> MSSDLVMPALGRPFTLGMLYDARREKLIPGFSLFGDETLQKYQSSNAQRSSEFKIVASDSTESKSSAMDIEASLGVSFLGGLVEVGGSAKYLNNTKKYQNQSRVTLKYKATTVYKQFTAPPGTVTVQETAITEKGLATHVVTSILYGANAFFVSDSDKVEDTNLQDIQGKMEAAIKKIPTISIEGSASVQLTDEEKSLASNLSCKFHGDFLLESLPTTFEDAVKTYQTLPTLIGEDGANSVPMKVWLAPLKSYNSKAQQLIQEINVSKVRRIHTTLEELHKLKRRANEAMDVKLVQRIPLIHDKISNFQQIFQDYMLTVQKKIAEKLPLVRAGTESEQSLQKIIDDRAQSPFSNEKVSKWLDAVEREIAVLKSCAGMVEGTQAKFVSNQTELDREVLVGKVKHAVCFIFTSVERNDPYLKVLSDYWESPPSNNAKDVAPSTEDKWCFSTEVVLKMQQRAQTFCDHVNDFEKSRNVGFFITALENGKFQGASIYYYKEGSLATQDFTFPRMPFVQGYKKRSDLLWYACDLTFDRNTINNWISLSDNDTFAASEHGKRQNYPKHPERFVSFNQVLCNEGLMGKHYWEVEWNGYIDVGIAYISIPRKEIDFASAFGYNTYSW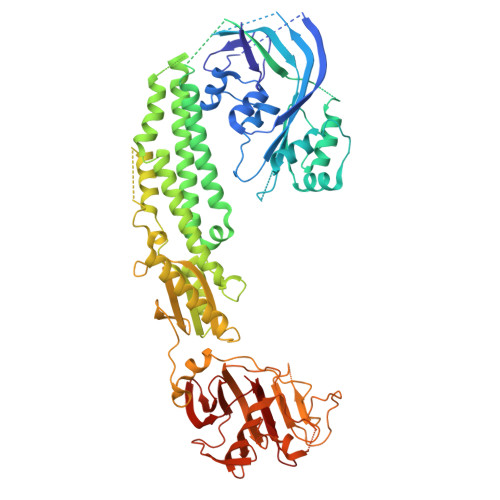VLSYNPKIGYIERHKKREYNVRAPNPGFKRLGLFLDWRYGSISFYAVSSDEVHHLHTFKTKFTEPVYPAFSIGPAGNHGTLRLL> SLRD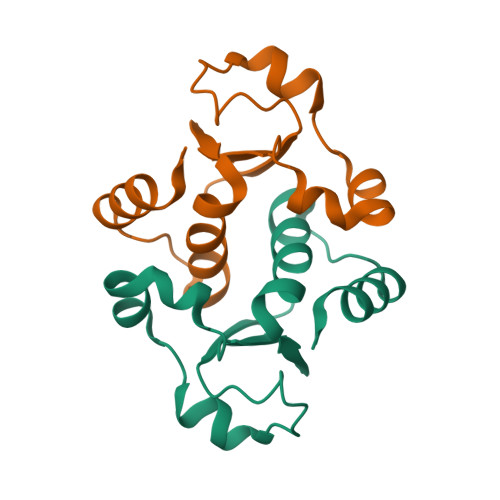LPSIAISLCGGLSDHREITKDAFLEQAVSYQQFADNPAIIDDPNLVVKVGNKYYNWTTAAPLLLAMQAFQKPLPKATVESIMRDKMP In most cells, the detoxification of sulfite by oxidation to sulfate (Equation 1) is catalyzed by sulfite oxidizing enzymes (SOEs). Here, we have investigated an electron transfer complex involving the periplasmic SorT sulfite dehydrogenase from the α-Proteobacterium Sinorhizobium meliloti, which represents a structurally uncharacterized type of SOE, and its electron acceptor, the c-type cytochrome SorU. In S. meliloti the SorT sulfite dehydrogenase is part of a sulfite detoxification system that is induced in response to the degradation of sulfur containing substrates such as the organosulfonate taurine. Electrons derived from sulfite oxidation are passed on to the SorU cytochrome, and likely then to cytochrome oxidase, as S. meliloti is capable of sulfite respiration.

Despite the dynamic nature of the SorT/SorU interaction, it was possible to co-crystallize SorT with SorU, resulting in the crystal structure of the SorT/SorU complex, where a single SorT/SorU entity is present per asymmetric unit, and the application of crystallographic 2-fold symmetry reveals a SorU/SorT2/SorU assembly. In the SorT/SorU complex, the SorU protein docks within a pocket adjacent to the SorT active site, with the heme cofactor located at the protein-protein interface. The shortest ‘edge-to-edge’ distance between the SorT Mo atom and the propionate group from the SorU heme c cofactor is 8.2 Å, which is well within the distance for fast electron transfer through the protein medium. The SorT/SorU complex interface shows significant charge complementarity, with the negative charge on SorU correlating with a concentration of positive charges at the SorU binding site on SorT. In addition to the electrostatic interactions that support the formation of the SorT/SorU complex, there are six hydrogen bonds found at the SorT/SorU protein-protein interface, as well as a salt bridge between the SorT active site residue Arg 78 and a propionate group of the SorU heme moiety. Specific structural adaptations of the SorU protein take place when the SorT/SorU assembly is formed. A surface loop on SorU (residues 82–93) moves away from the SorT/SorU complex interface, leading to a reorientation of the heme ligand residue Met 87 so that a different Met 87 rotamer coordinates the iron in the SorU structures within and outside of the complex. This change in the structure of SorU is required to allow a Mo-heme edge-to-edge distance of ‘closest approach’ of ca. 8 Å within the SorT/SorU assembly. The structural change in SorU indicates that an ‘induced fit’ mechanism is responsible for the formation of a productive SorT/SorU electron transfer complex. Within the SorT/SorU complex, the SorU protein shows a significantly increased average atomic temperature factor (reflecting significant flexibility) relative to the structure of the SorT protomer (1.5 versus 0.9 Å2, respectively).

> SKETKPLPDYVAWKDADALIVHSDKTLETKRSEFGTSIITPEEKLYIRNNVNTPPESILADRDGWKVEISGVKEPRTLTVAELKTLGLVTAATVLQCSGNGRKYFKDQLTGDQKMSGTPWTVGAAGCVIWSGVPLKAVVDALGGPAEGARFITGTGGEELPAGLDPKLLVVERSVPISNLDNVILAWEMNGRPLSLAHGGPLRMVVPGYSGVNNIKYVKAVAMTEVETDAKIQKTSYRVHALGEKGSPDQPSVWEQPVKSWITTPHEAAKAGQVQIAGVAFGGMNACKSVEVSVDGGQTWQEAEFIGPDLGRFAWRVFALSADLARGTYTLVSRATDTEGNVQPEETEMNGAGYGHNGWRAPAVKLTVA;> MEEDKLALGREIFLERSEPQCALCHTLADAEAVGEVGPNLDELKPDAERVNTAVTNGIGPMPANEILTDEEIEAVALYVSTVAGKAKNSSSVDKLAAALEHHHHHH5-[4-[[(1~{R})-1-[3-[bis(fluoranyl)methyl]-2-fluoranyl-phenyl]ethyl]amino]-2-methyl-6-morpholin-4-yl-7-oxidanylidene-pyrido[4,3-d]pyrimidin-8-yl]pyridine-2-carbonitrile 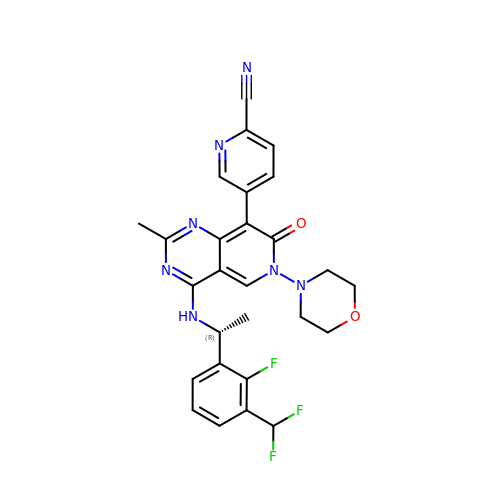| C27 H24 F3 N7 O2 | HRMKBFIINYRRDO-OAHLLOKOSA-N> MGFAWWGRTVYQFRYIVIGVMVALCLGGGVYGISLGNHVTQSGFYDEGSQSVAASLIGDEVYGRDRTSHVVAILTPPDDKKVTDKAWQKKVTEELDQVVKDHEDQIVGWVGWLKAPDTTDPTVSAMKTQDLRHTFISIPLQGDDDDEILKNYQVVEPELQQVNGGDIRLAGLNPLASELTGTIGEDQKRAEVAAIPLVAVVLFFVFGTVIAAALPAIIGGLAIAGALGIMRLVAEFTPVHFFAQPVVTLIGLGIAIDYGLFIVSRFREEIAEGYDTEAAVRRTVMTSGRTVVFSAVIIVASSVPLLLFPQGFLKSITYAIIASVMLAAILSITVLAAALAILGPRVDALGVTTLLKIPFLANWQFSRRIIDWFAEKTQKTKTREEVERGFWGRLVNVVMKRPIAFAAPILVVMVLLIIPLGQLSLGGISEKYLPPDNAVRQSQEQFDKLFPGFRTEPLTLVMKREDG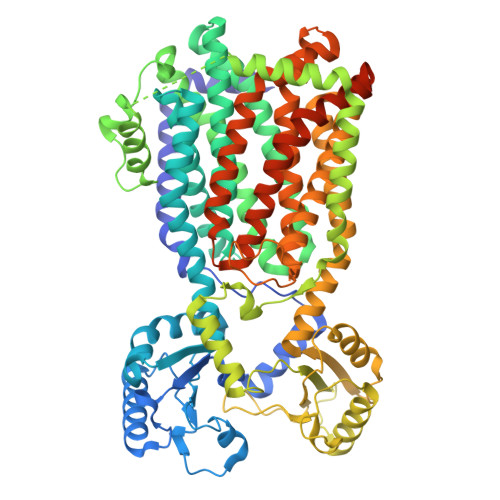EPITDAQIADMRAKALTVSGFTDPDNDPEKMWKERPANDSGSKDPSVRVIQNGLENRNDAAKKIDELRALQPPHGIEVFVGGTPALEQDSIHSLFDKLPLMALILIVTTTVLMFLAFGSVVLPIKAALMSALTLGSTMGILTWMFVDGHGSGLMNYTPQPLMAPMIGLIIAVIWGLSTDYEVFLVSRMVEARERGMSTAEAIRIGTATTGRLITGAALILAVVAGAFVFSDLVMMKYLAFGLLIALLLDATIIRMFLVPAVMKLLGDDCWWAPRWMKRVQEKLGLGETELPDERKRPTVRESETDQRENLYFQ MpPA14 (Marinomonas primoryensis PA14 domain) lectin is a domain of a 1.5-MDa adhesin responsible for a symbiotic bacterium-diatom interaction in Antarctica. Bioinformatic analyses indicated the presence of an ∼20-kDa domain near the C terminus of MpIBP that is a member of the PA14 family, which is a carbohydrate-binding lectin module widely distributed across several kingdoms of life. PA14 domains share a β-sandwich fold and the presence of two consecutive aspartate residues in a cis peptide linkage (DcisD). The DcisD motif coordinates a Ca2+ ion that is directly involved in binding polar vicinal hydroxyl groups of various carbohydrates.

We further analyzed the crystal structures of MpPA14 in complex with three pentoses, l-arabinose, ribose, and 2-deoxy-ribose, as well as inositol, which has an unusual 6-carbon saccharide ring without an endocyclic oxygen. These four carbohydrates bound MpPA14 more weakly than glucose and mannose. Crystal structures showed that MpPA14 selects the pyranose form of pentoses for binding. As pentoses have a higher percentage of furanose present in the conformational equilibria than do hexoses, selectivity for the more thermodynamically stable pyranoses might contribute to the weaker affinity of pentoses toward the lectin. For instance, despite l-arabinose existing in solution predominantly in the pyranose form at 25°C (57% α-arabinopyranose versus 30.5% β-arabinopyranose), only the α-anomer complexes MpPA14 via its 1,2-diol. The same rationale can be used to explain the even weaker affinity of ribose and its derivative 2-deoxy ribose for MpPA14 (se Fig. S5B and C in the supplemental material).

> KAQDDSTPDSLFAGLVGEYYGTNSQLNNISDFRALVDSKEADATFEAANISYGRGSSDVAKGTHLQEFLGSDASTLSTDPGDNTDGGIYLQGYVYLEAGTYNFKVTADDGYEITINGNPVATVDNNQSVYTVTHASFTISESGYQAIDMIWWDQGGDYVFQPTLSADGGSTYFVLDSAILSSTGETPYTT> MATQMQQRDNGEETLANIKHSARSELKDMNVSGLAGINIQAGGYDLTGLSLTDELIAQGLSNVGLLPFEHSRVVLELAEAITVTANNTDMGGSGQYCEQGAWRAWLHVGLNMAKHHVRIRSSAAMDFGTHRMMACDPASLDASTISAMSRNVTTATMNAVSREMKAMKALAAGRSRMSQSDIADNNDCRGFAFGVLSRMVMHNSARRHGVVNGRLQELGENDASTADTYLTWELACAHGKGEVAITPVPAAWLDPEAQLTGRERVFSEALARLVDPDVGCVHVKIDGVTQNAAENARVHYATRPDPMSWLDDNTGLSADSNAGRISGEHYTLWKGRHSKVHLTIQLKQLYHRMSTTAATAEPRADSIVYYLKGFEGLGACAEFLLANSRFGHHSFLPGVFGVTADVHEAAYAQNQALFLAGIGDRMPPATFTKAQLATATYALMRRYDISERTCHFAITTIGHMVAQTAVRDLNNGSLSPLPFRVNLSPFLVQGVQFWDMNDTEGSVSVHDMGIGKELLTATYALGAMASLAHVCEQGGTGEEMSAIEVSRFTDVHTVATDLFRKVVMTELGDLKLRGSEVTHSSQEALFAQKMKAVWSSMAEGSTRLYNLNQAYGPFVDVQLARIRSSFVRDIGASRQMMDASALIKHAQNVTYDWPQNESGCPVQFIALPVPSTITHYATPAIGTERWFATTRLNAAGSKVISEIRWTNGLNSDDRAGVHVFAYGRSTIVSSPLGCAEAMAAMVIAGEHKVVRRHTSIARAQSARTANIVAGAVLGARNGDMMTIIRPSTSVASSAVHLRGYIPMAAMNMLPITDGDCDLVVADTRTRPGRMSTSPEAHRRGVLASDYHVDIATDGNIRHVAREVYTVADIPTVSERVSGLALRPYERSCVRDASTLHSMLCGAVPLLYGGGEPMKLGDNTPVTNRQALRPPEYNRNPALRMPARFQMGTTACAFTKALGDVRAQMELREGDVVTEEVTEPDTTIVPQGSITERVVVGEMTEALIMADQPMFDQDVVQNIMYNSPGIRGTERANIQAELMAAKDWPSILQATAKSSHGDIASAKTPYDLIKACKVDWSKVKGETQLKLIMNKIHPEYMTLSRAISAQVDARIVPNVPKSAMSTLLFWACATDMGLHTAVMANLAGLQRTTGFKGGIVYDLEGGANWPATDVRARIIEGWNAHARRIAQSGLISRDLTVMKIQHDMNADDIMALPAHIGDSWVLTIGELTANIATDEQSVAYAKDAQSAYYAIDRLRRLVAGREEGVDEILSKAEVMARVLAENKGLADDQALYHREWNRRTMAYVYMTTYLGSLDVEARLGVVSDDAYAERRAEWKAERAKLAVPAVSGQGQGRR;> MSAPSDQSQETRSPTSVGNTVAADVQTSVHDKPTGELKGSDGTGIHEATGLPIDKRGEVPTVQLERTAESIAKMMDLLRSEKFTAAAADAKLMLQQEFQNIVACAKNAPQMTVNAGRFYLGCNSTTAIIAGDTADGYEIEYSGKRIEGQCVVALEPLTITLSGSTSSTQDNSDSAKLFALAVSQVWGGASTVGIVAPMLQTVAQEQTFRARVERDSGFQHHAALTTVVTTIVGWLMHVGDSAAKRSRDGWLDHQTDFAVKGMLTPHIASGMDWAGVQTYSASAMETTTDRVRADYAGRMVVHSTLRKQTLRSRGTGDTTETENSGRYLLALPKCDAGVAAAALALTWGKPKLGGAGHANLTAVMSEAGVGYITGVNGTRATPHADTVFGREELVYLLGFALRHMADAQEQVIRNVLAQVASLFRPAACSAHEWMNVHGALMPKVSRPMNEPAFREVWNVANSSSDLQMIDRDKLNGEHFLRQLAQQITVNCTGTAMAIYQAVLAGPTGITDGDTTRLQKDLYHHLFQYATTTYADGVQVMQANTRMANKMVPPVNALAAWGLGSSMDSFTGPHCAYYFGLADAADGCFYSTTTGRTLSVYAVDVNHTSSDSYLAMAQLEPGLIATATGTGSTITTNVEAAGVVDGGLVTEGHVSLYTTISAQWNGLQREVYNWLLWHACKTEDSSHADIVGAEEVKSAVEWLSSNSVEAHRFRSSAGLGATEAAGSPGRRAWRLHHYDGQIFSNVIADTERHPYMR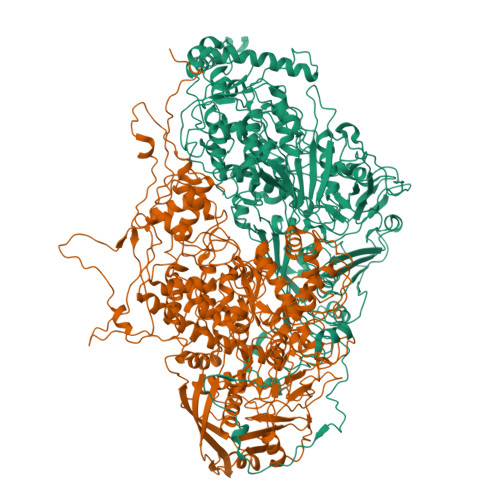RLYTPSELRDARNDLFVVDRIWKIVMAMRAQLMLISVQEDGGRHQHSKHYFGEAAAIGVMGHGFTNLFAYCASTVHGGREARLISNCTDTPMYKKEANDLVPPMMKVAQLSTLLAHGGAWCNAVNMGGNSTSIGLSILGDGTMPLQTVPWTVNEITYLSEEGARHGIEAIIDTNGSVSVKVKMTMLEPRQRFCLYDDNKTSSYITAQESRTATYVTLKLGGTKNANTISGLVAHDYKLATTILASTYDKGRKTGLTLEDLQKVGGITGGQGMTGRGGGSSSGRGGRGRGGSSTGGAETIGDSE> XXXXXXXXXXXXXMSSEDIIYDPQFKPVQGIYENRLRQFIDTGGDYHDLNLPKFYDKKRISLDHDHVKVWWYQVSFERGSSPVSPDKRPSWKSIIERDKKGELEFRE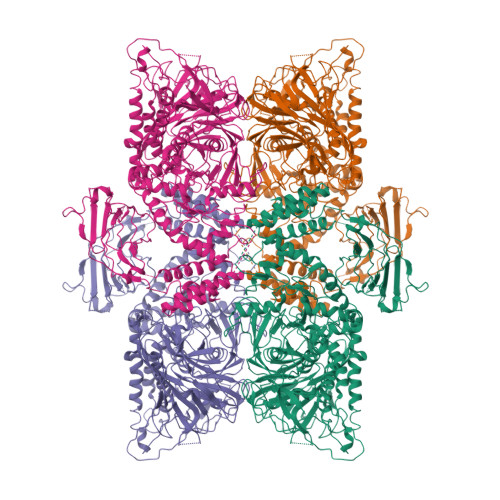ANINQPFGPSWSTTWFKVKISLPEDWVKSNEQLLFQWDCSNEGIVIDPKTLIPVTAFSGGERTEYVLPKTSDGKHFFYIEAGNNGMFGCGAGSTINPPDDNRFFHLRKADIVWPDLDARALYIDFWMLGDAARELPGDSWQKHQARQLGNAVMNLFDPNDRSSVRKCRELLQREYFDSFLESSKVYEQGESQVLTNVYGIGNCHIDTAWLWPFAETRRKIVRSWSSQCTLMDRFPEYKFVASQAQQFKWLLEDHPEFFNKVLIPKIQQSQFFAVGGTWVENDTNIPSGESLARQFFFGQRFFLKHFGLKSKIFWLPDTFGYSSQMPQLCRLSGIDKFLTQKLSWNNINSFPHSTFNWAGIDGSQLLTHMPPGNTYTADSHFGDVLRTAKQNKTPEYYGSGLMLYGKGDGGGGPTEEMLQKMRRIRSMNNRNGNVIPKLQVGITVDEFYDDILKRTNQGHDLPTWSGELYFEFHRGTYTSQAQTKKLMRLSEIKLHDLEWIAAKTSVLYPDSYKYPSKQINELWENVLLCQFHDVLPGSCIEMVYKYEAVPMLHNVVKECTSLIDKTVQFLQSQSKADLVEMRTLTWSKPEKVSEECSLNGSYTSSVTGYDDYIVLANGKLKVIICKKTGVITSITDETLGVEYLDTEHGRNKLGANQFVIYDDKPLGWQAWDTELYSVNQYKYVTKPKKVQVSCNTKEKCAVEVIFQISEKCKIKSVISLNATAVTDAKLSKVDISTTVENWDARNKFLKVEFPVNIRNDFASYETQFGITKRPTHYNTSWDVAKFEVCHHKFADYSEYSKGVSILNDCKYGFSTHGNLMRLSLLRSPKAPDAHADMGTHEIKYAIYPHRGALSSDTVKLAHEFNYCFKYKLPKDIGMNFDDIISISGDENVILSNIKRGEDDSAVKSNYSLNPRDEQSIVVRVYESLGGESFASLNTTLNLKRIEKVDNLEMKVYKSLTATRDESNHAINRIPIKLRPFEIASFRLYF>MSISISYSTTYSGWTVADYLADWSAYFGDVNARPGQVVDGSNTGGFNPGPFDGSQYALKSTASDAAFIAGGDLHYTLFSNPSHTLWGKLDSIALGDTLTGGASSGGYALDSQEVSFSNLGLDSPIAQGRDGTVHKVVYGLMSGDSSALQGQIDALLKAVDPSLSINSTFDQLAAAGVAHATPAAAAAEVGVVG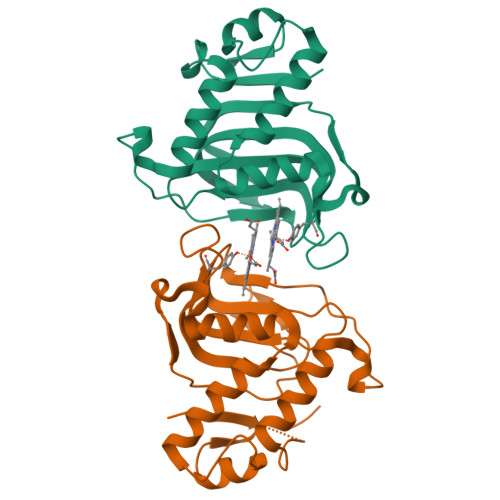VQELPHD[2x]>TSNVITQDLPIPVASRGFADIVGFGLDGVVIGRNAVNLQPFLAVKNFAQNAGGWLTTKHVRLIADTTGTGKGDIVGFGNAGVYVSVNNGKN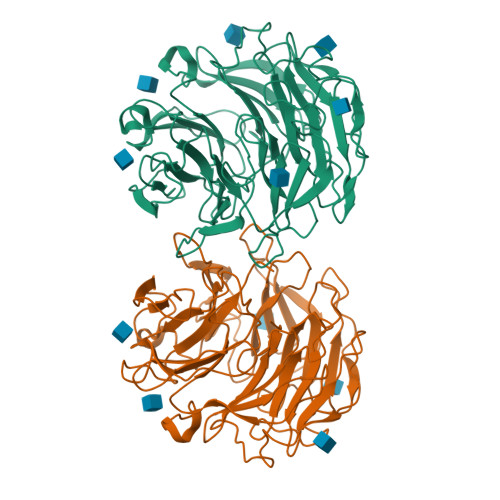TFADPPKMVIANFGYDAGGWRVEKHLRYLADIRKTGRADIIGFGEKGVLVSRNNGGLNFGPATLVLKDFGYDAGGWRLDRHLRFLADVTGNGHLDIVGFGDKHVFISRNNGDGTFAPAKSVIDNFCIDAGGWKIGDHPRFVADLTGDGTADIIGCGKAGCWVALNNGGGVFGQVKLVINDFGTDKGWQAAKHPRFIADLTGNGRGDVVGFGNAGVYVALNNGDGTFQSAKLVLKDFGVQQGWTVSKHRRFVVDLTGDGCADIIGFGEKETLVSYNDGKGNFGPVKALTNDFSFSGGKWAPETTVCWMANLDSSRH[2x]> 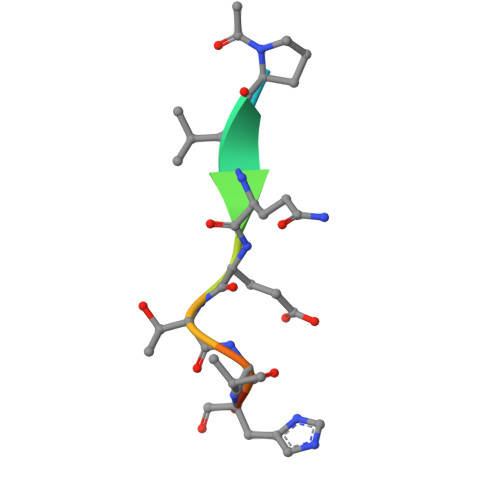XPVQETLHGC>SLSPAVQTFWKWLQEEGVITAKTPVKASVVTEGLGLVALKDISRNDVILQVPKR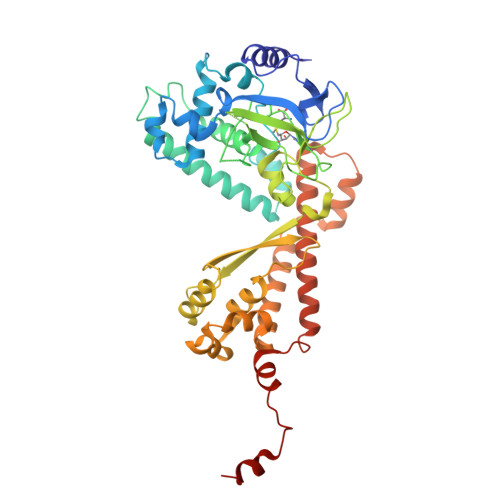LWINPDAVAASEIGRVCSELKPWLSVILFLIRERSREDSVWKHYFGILPQETDSTIYWSEEELQELQGSQLLKTTVSVKEYVKNECLKLEQEIILPNKRLFPDPVTLDDFFWAFGILRSRAFSRLRNENLVVVPMADLINHSAGVTTEDHAYEVKGAAGLFSWDYLFSLKSPLSVKAGEQVYIQYDLNKSNAELALDYGFIEPNENRHAYTLTLEISESDPFFDDKLDVAESNGFAQTAYFDIFYNRTLPPGLLPYLRLVALGGTDAFLLESLFRDTIWGHLELSVSRDNEELLCKAVREACKSALAGYHTTIEQDRELKEGNLDSRLAIAVGIREGEKMVLQQIDGIFEQKELELDQLEYYQERRLKDLGLCGENGDILENLYFQ[3x]> KDITDKNQSIDSGISSLSYNRNEVLASNGDKIESFVPKEGKKAGNKFIVVERQKRSLTTSPVDISIIDSVNDRTYPGALQLADKAFVENRPTILMVKRKPININIDLPGLKGENSIKVDDPTYGKVSGAIDELVSKWNEKYSSTHTLPARTQYSESMVYSKSQISSALWVNAKVLENSLGVDFNAVANNEKKVMILAYKQI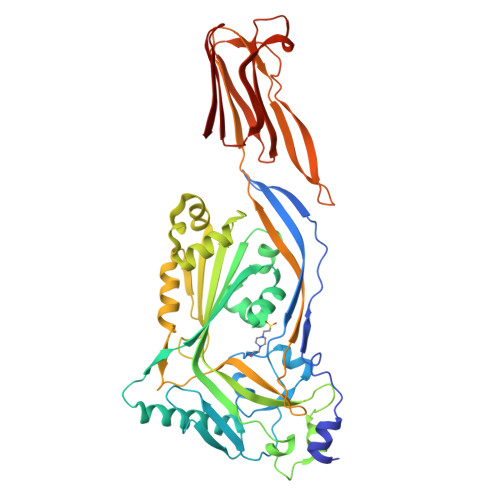FYTVSADLPKNPSDLFDDSVTFNDLKQKGVSNEAPPLMVSNVAYGRTIYVKLETTSSSKDVQAAFKALIKNTDIKNSQQYKDIYENSSFTAVVLGGDAQEHNKVVTKDFDEIRKVIKDNATFSTKNPAYPISYTSVFLKDNSVAAVHNKTDYIETTSTEYSKGKINLDHSGAYVAQFEVAWDEVSYDKEGNEVLTHKTWDGNYQDKTAHYSTVIPLEANARNIRIKAREATGLAWEWWRDVISEYDVPLTNNINVSIWGTTLYPGSSITYN>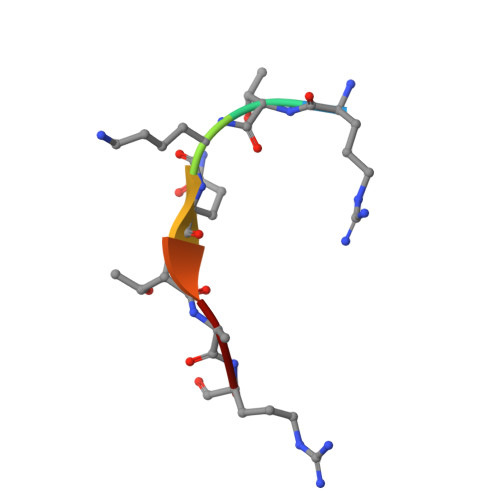 RTKQTAR>[4x]MERPEPELIRQSWRAVSRSPLEHGTVLFARLFAL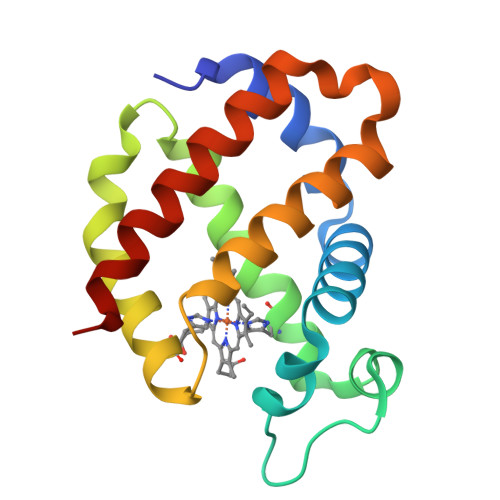EPDLLPLFQYNGRQFSSPEDSLSSPEFLDHIRKVMLVIDAAVTNVEDLSSLEEYLASLGRKHRAVGVKLSSFSTVGESLLYMLEKSLGPAFTPATRAAWSQLYGAVVQAMSRGWDGE> MKVYKDVFTNDEVCSDSYNQEDPFGIADFREIAFEVKSNKRIKGNDDYGIADNSEEAVDGMGADVEQVIDIVDSFQLTSTSLSKKEYSVYIKNYMQKILKYLEEKKPDRVDVFKTKAQPLIKHILTNFDDFEFYMGESLDMDAGLTYSYYKGEEVTPRFVYISDGLYE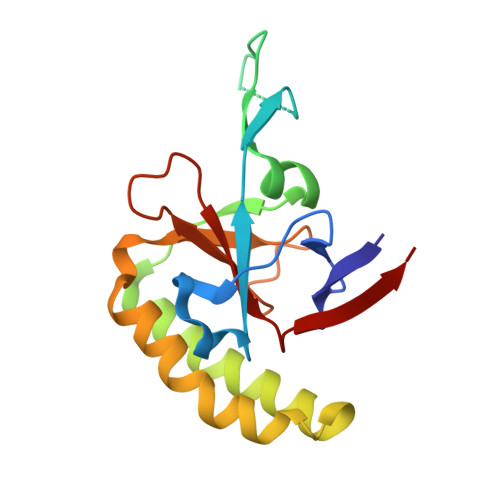EKF> YDPIHEYVNHELRKRENEFSEHKNVKIFVASYNLNGCSATTKLENWLFPENTPLADIYVVGFQEIVQLTPQQVISADPAKRREWESCVKRLLNGKCTSGPGYVQLRSGQLVGTALMIFCKESCLPSIKNVEGTVKKTGLGGVSGNKGAVAIRFDYEDTGLCFITSHLAAGYTNYDERDHDYRTIASGLRFRRGRSIFNHDYVVWFGDFNYRI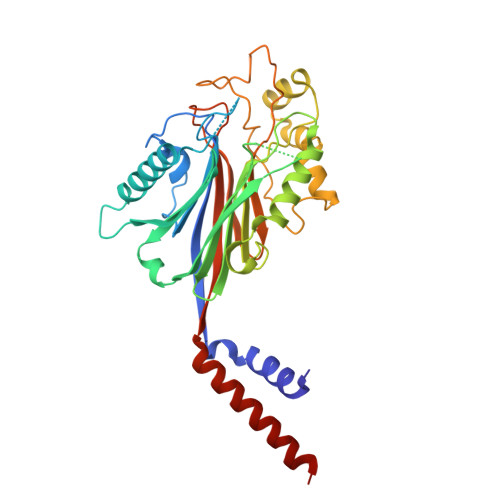SLTYEEVVPCIAQGKLSYLFEYDQLNKQMLTGKVFPFFSELPITFPPTYKFDIGTDIYDTSDKHRVPAWTDRILYRGELVPHSYQSVPLYYSDHRPIYATYEANIVKVDREKKKILFEELYNQRKQEVRDASQTS trans-4-({[3-(furan-3-yl)-2,4-dihydroindeno[1,2-c]pyrazol-6-yl]methyl}amino)cyclohexanol | C21 H23 N3 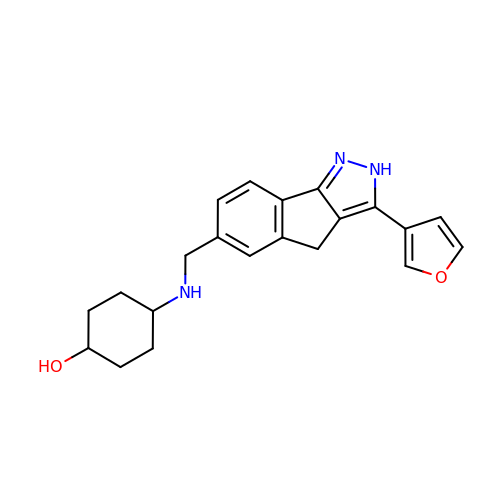O2 | MQYHCTJCBXXBCX-QAQDUYKDSA-N> MSFFAGKLNNKSILSLRRGSGGDTNQHINPDSQTIFHSDMSHVIITETHSTGLRLDQGAGDYYWSEMPSRVTQLHNNDPNRVVLTEIEFSDGSRHMLSGMSMGVGAKAYGIINPQIMSQGGLKTQITASADLSLDVGYFNTGTSGTIPQKLRDGTGCQHMFGAFSGRRGFASSAMYLGGAALYKSAWSGSGYVVADAGTLTIPSDYVRHPGARNFGFNAIYVRGRSCNRVLYGMEGPNYTTGGAVQGASSSGALNFTYNPSNPESPKYSVGFARADPTNYAYWESMGDPNDSANGPIGIYSEHLGIYPSKITWYVTNLVYNGSGYNIDGGLFNGNDIKLSPREFIIKGVNVNNTSWKFINFIEKNFNVGNRADFRDVGCNLSKDSPSTGISGIATFGLPTTESNNAPSIKGGNVGGLHANVVSIYNFLPSASWYVSSNPPKIGNNYGDVWSENLLPLRLLGGSGSTILSGNIVFQGNGSVHVGTVGLDLNSSRNGAIVCTMEFIDDTWLSAGGIGCFNPTEMLSQGAEYGDS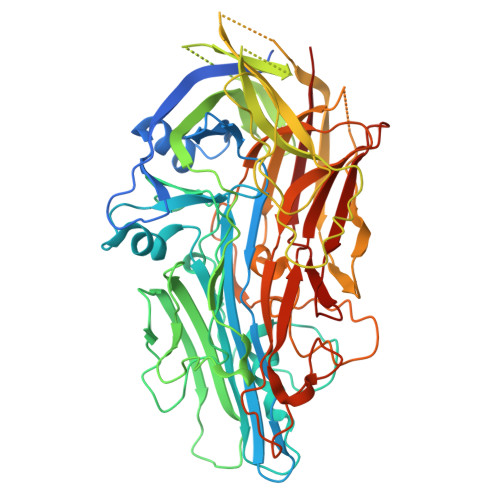RFRIGGNTINKKLHQILSLPAGEYVPFFTIKGTVVNACKLQAAAYNPTPYWVSGLPGSVGQTGYYTLTYYMRNDGNNNISIWLDSSMSNIIGMKACLPNIKLIIQRLTHHHHHH> MKLLKILSLVCLSISIGACAEHSMSRAKTSTIPQVNNSIIDQNVQALFNEISADAVFVTYDGQNIKKYGTHLDRAKTAYIPASTFKIANALIGLE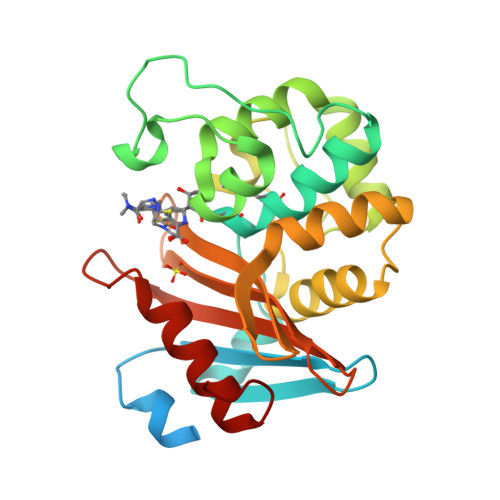NHKATSTEIFKWDGKPRFFKAWDKDFTLGEAMQASTVPVYQELARRIGPSLMQSELQRIGYGNMQIGTEVDQFWLKGPLTITPIQEVKFVYDLAQGQLPFKPEVQQQVKEMLYVERRGENRLYAKSGWGMAVDPQVGWYVGFVEKADGQVVAFALNMQMKAGDDIALRKQLSLDVLDKLGVFHYL> YGPKGPKGPKGKPGPDGDPGDPGDPGPKGPK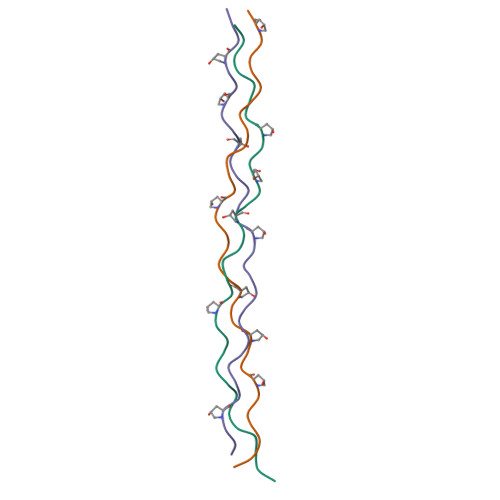G;> YGPDGDPGDPGDPGPDGKPGPDGPDGPDGDPG;> YGKPGPEGPEGPKGKPGPKGKPGKPGKPGKA> MSSDSFQRQLVQRTNTLNSSIDNATLTILSRFQDILDIAINEGKDKYTVAPEVYQIECHTVSMVRAVEQL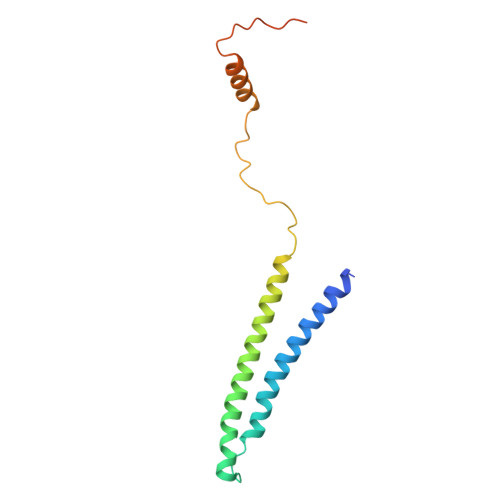LDVSRQIKSYWLTNSLSTSFPTVDYSEPDLEKVKRTLTKLQNHLLEVSLIEPEASETTEAPTVSDT> GSMTSPRNCLRFTLLGCGSSPGVPRINGDWGKCDPKNPKNRRRRASLLVERYDAEGNNTVVVIDTGPDFRMQMIDSGVHMLDAAVYTHPHADHIHGIDDLRTYVVDNGRLMDVYANRLTRNRLYDTFGYCFETPVGSSYPPILSMHDIAPETPFSIEGAGGAIRFEPFSQVHGDIESLGFRIGSVVYCTDVSAFPEQSLQYIKDADVLIIGALQYRPHPSHFSLGEALEWIEKLSPKRAILTHMHVPLDYETVMRETPHHVEPGYDGLRFEVAV

Here, we report the high-resolution structure of BrabA.11339.a, a structural genomics target that entered the pipeline as a ‘β-lactamase-like protein’. β-Lactamases break down β-lactam antibiotics such as penicillin and lead to the resistance of pathogens to antibiotics. BrabA.11339.a assumes a metallo-β-lactamase-like fold with two central β-sheets. As a very typical feature of β-lactamase-like proteins and the phosphodiesterase protein family, a two-metal center is present in the active site of BrabA.11339.a. It therefore seems likely that BrabA.11339.a is a GTP/ATP or GDP/ADP hydrolase.

In order to analyze the metal center in more detail, diffraction data sets with high multiplicity were collected at long X-ray wavelengths from the ligand co-crystals: in-house at λ = 1.5418 Å and at the synchrotron at λ = 1.3476 Å. For both long-wavelength data sets and the Se-edge data set strong anomalous Fourier peaks can be observed for the two active-site metals. Each of the peaks is about four times as strong as the signal for potassium. The anomalous signal for Ni2+ is strong at the Se edge and at 1.3476 Å; however, it is low at 1.5418 Å. Manganese is the only metal in question that has a significant anomalous signal at all three wavelengths. Therefore, the dinuclear center of BrabA.11339.a can be assigned as two manganese ions with a high degree of confidence. In order to confirm the binding of nucleotides, crystals were grown in the presence of GMPPNP and AMPPNP. In both cases, however, very solid electron density could be observed for GMP and AMP, respectively. The γ-­phosphate groups of GMPPNP or AMPPNP, which had been added during crystal growth and had been supplemented for a short soak in the cryobuffer, are nonhydrolyzable; the β-phosphate groups, however, can be hydrolyzed. It can be assumed that BrabA.11339.a is able to hydrolyze AMPPNP and GMPPNP between the α-phosphate and the β-phosphate to AMP or GMP, respectively.>MRLHPRTEAAKESIFPRMSGLAQRLGAVNLGQGFPSNPPPPFLLEAVRRALGRQDQYAPPAGLPALREALAEEFAVEPESVVVTSGATEALYVLLQSLVGPGDEVVVLEPFFDVYLPDAFLAGAKARLVRLDLTPEGFRLDLSALEKALTPRTRALLLNTPMNPTGLVFGERELEAIARLARAHDLFLISDEVYDELYYGERPRRLREFAPERTFTVGSAGKRLEATGYRVGWIVGPKEFMPRLAGMRQWTSFSAPTPLQAGVAEALKLARREGFY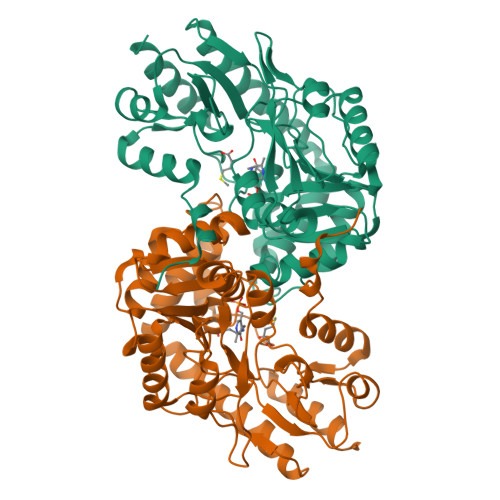EALREGYRRRRDLLAGGLRAMGLRVYVPEGTYFLMAELPGWDAFRLVEEARVALIPASAFYLEDPPKDLFRFAFCKTEEELHLALERLGRVVNSPREAEGGAVSG[2x]> MGSH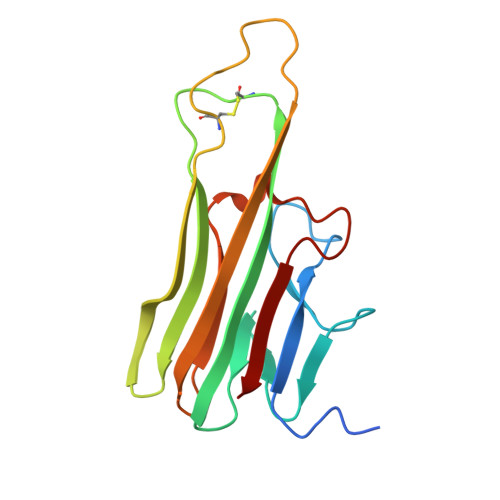HHHHHRTPSDKPVAHVVANPQAEGQLQWLNRRANALLANGVELRDNQLVVPSEGLYLIYSQVLFKGQGCPSTHVLLTHTISRIAVSYQTKVNLLSAIKSPCQRETPEGAEAKPWYEPIYLGGVFQLEKGDRLSAEINRPDYLLFAESGQVYFGIIAL> ADKELKFLVVDDFSTMRRIVRNLLKELG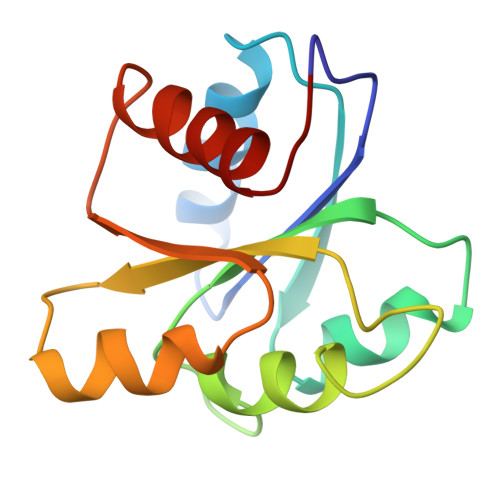FNNVEEAEDGVDALNKLQAGGFGFIICDWNMPNMDGLELLKTIRADSAMSALPVLMVTAEAKKENIIAAAQAGASGYVVKPFTAATLEEKLNKIFEKLGM>MTGMSREEVESLIQEVLEVYPEKARKDRNKHLAVNDPAVTQSKKCIISNKKSQPGLMTIRGCAYAGSKGVVWGPIKDMIHISHGPVGCGQYSRAGRRNYYIGTTGVNAFVTMNFTSDFQEKDIVFGGDKKLAKLIDEVETLFPLNKGISVQSECPIGLIGDDIESVSKVKGAELSKTIVPVRCEGFRGVSQSLGHHIANDAVRDWVLGKRDEDTTFASTPYDVAIIGDYNIGGDAWSSRILLEEMGLRCVAQWSGDGSISEIELTPKVKLNLVHCYRSMNYISRHMEEKYGIPWMEYNFFGPTKTIESLRAIAAKFDESIQKKCEEVIAKYKPEWEAVVAKYRPRLEGKRVMLYIGGLRPRHVIGAYEDLGMEVVGTGYEFAHNDDYDRTMKEMGDSTLLYDDVTGYEFEEFVKRIKPDLIGSGIKEKFIFQKMGIPFREMHSWDYSGPYHGFDGFAIFARDMDMTLNNP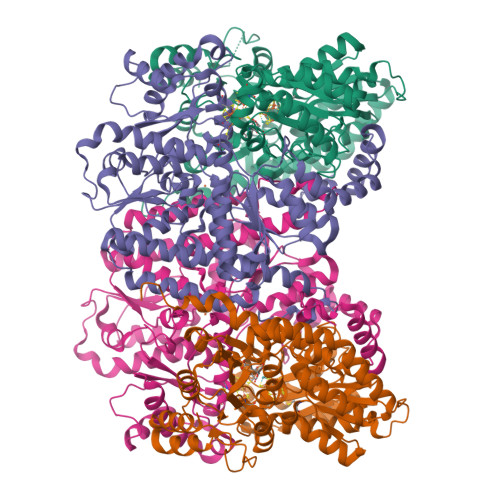CWKKLQAPWEASEGAEKVAASA[2x];>[2x]MSQQVDKIKASYPLFLDQDYKDMLAKKRDGFEEKYPQDKIDEVFQWTTTKEYQELNFQREALTVNPAKACQPLGAVLCALGFEKTMPYVHGSQGCVAYFRSYFNRHFREPVSCVSDSMTEDAAVFGGQQNMKDGLQNCKATYKPDMIAVSTTCMAEVIGDDLNAFINNSKKEGFIPDEFPVPFAHTPAFVGSHVTGWDNMFEGIARYFTLKSMDDKVVGSNKKINIVPGFETYLGNFRVIKRMLSEMGVGYSLLSDPEEVLDTPADGQFRMYAGGTTQEEMKDAPNALNTVLLQPWHLEKTKKFVEGTWKHEVPKLNIPMGLDWTDEFLMKVSEISGQPIPASLTKERGRLVDMMTDSHTWLHGKRFALWGDPDFVMGLVKFLLELGCEPVHILCHNGNKRWKKAVDAILAASPYGKNATVYIGKDLWHLRSLVFTDKPDFMIGNSYGKFIQRDTLHKGKEFEVPLIRIGFPIFDRHHLHRSTTLGYEGAMQILTTLVNSILERLDEETRGMQATDYNHDLVR>MAEREFDMTIEEVTIKVAPGLDYKVFGFNGQVPGPLIHVQEGDDVIVNVTNNTSLPHTIHWHGVHQKGTWRSDGVPGVTQQPIEAGDSYTYKFKADRIGTLWYHCHVNVNEHVGVRGMWGPLIVDPKQPLPIEKRVTKDVIMMMSTWESAVADKYGEGGTPMNVADYFSVNAKSFPLTQPLRVKKGDVVKIRFFGAGGGIHAMHSHGHDMLVTHKDGLPLDSPYYADTVLVSPGERYDVIIEADNPGRFIFHDHVDTHVTAGGKHPGGPITVIEYDGVPVDDWYVWKDK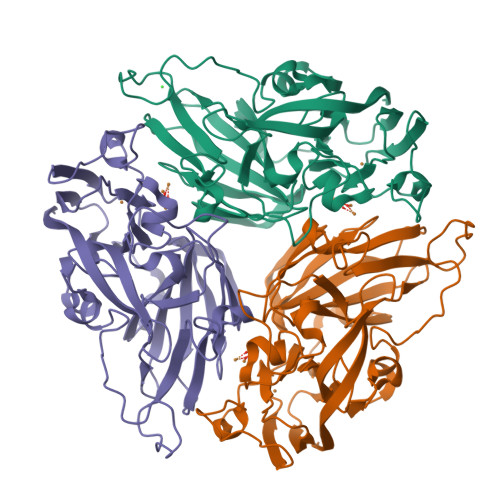DYDPNFFYSESLKQGYGMFDHDGFKGEFEQRQRRPGRKLAAALEHHHHHH[3x]>XTYSITLRVFQRNPGRGFFSIVEKTVFHYANGGTWSEAKGTHTLTMGGSGTSGVLRFMSDKGELITVAV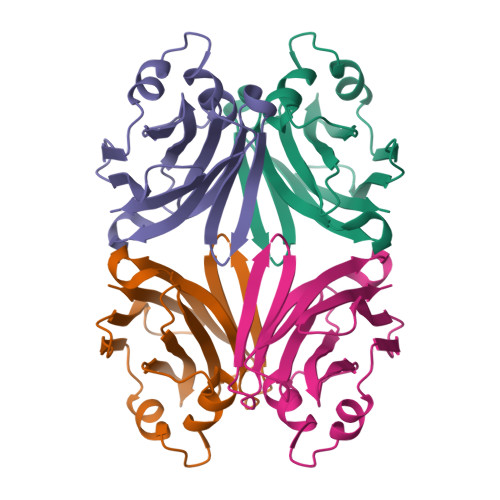GVHNYKRWCDVVTGLKPEETALVINPQYYNNGPRAYTREKQLAEYNVTSVVGTRFEVKYTVVEGNNLEANVIFS[2x]> MALMTWTAAEFGTNVGFADDQHKTIFDMVNKLHDTAATGNRSEIGKQLDALIDYVVMHFKSEETEMQKKGYADFAAHKAEHDKLVGVCADLQKKFHAGEAEVNQDTTRFVRDWAVN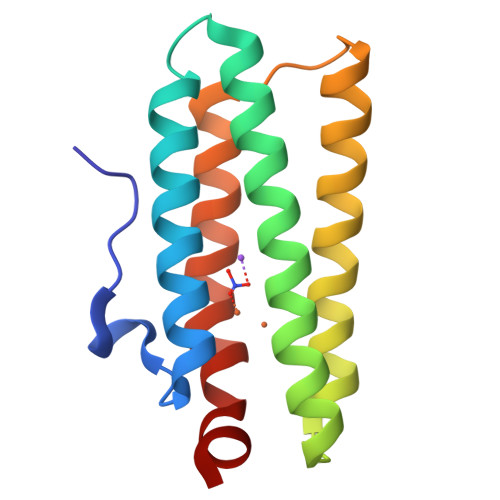HIPKVDKLYGPCLSA>MSLDPEDVYDGGYGSKHSPVQLRI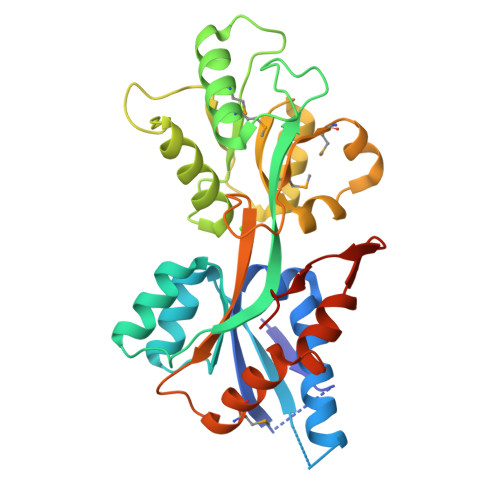GNGGAGQSGLVKELADAFIKSKVDSGSAPFKVAWYKSDTTVTINYLKDGIVDVGITYSPVAERISIKHGISESPSYYAFRDHFMLIGPPSNPAKLSGDSDIADMFSKMHDAAEAGNTKPPVRFLSRYDKSATNIKEAELWLSIGQVPWATAYSTWYHQYITFPIQALTAAILLREYTITDYGTYLSIPRGLRDQMVIYKKGTNDADDPLLNPAHLLVGARAKNAEMAKEFAKWLVSKEGGQKVIEGFKKDGQQLYSPAPYRHEGHHHHHH[4x]> ENALLRYLLDK;> KPEPTDEEWELIKTVTEAHVATNAQGSHWKQKRKFLPEDIGQAPIVNAPEGGKVDLEAFSHFTKIITPAITRVVDFAKKLPMFCELPCEDQIILLKGCCMEIMSLRAAVRYDPESETLTLNGEMAVTRGQLKNGGLGVVSDAIFDLGMSLSSFNLDDTEVALLQAVLLMSSDRPGLACVERIEKYQDSFLLAFEHYINYRKHHVTHFWPKLLMKVTDLRMIGA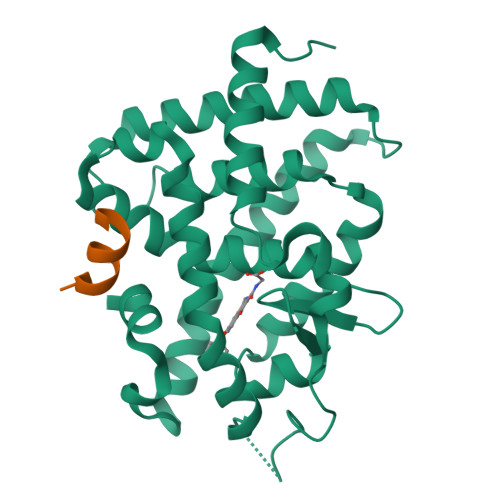CHASRFLHMKVECPTELFPPLFLEVFE> GPMGNGMNKILPGLYIGNFKDARDAEQLSKNKVTHILSVHDSARPMLEGVKYLCIPAADSPSQNLTRHFKESIKFIHECRLRGESCLVHCLAGVSRSVTLVIAYIMTVTDFGWEDALHTVRAGRSCANPAVGFQRQLQEFEKHEVHQYRQWLKE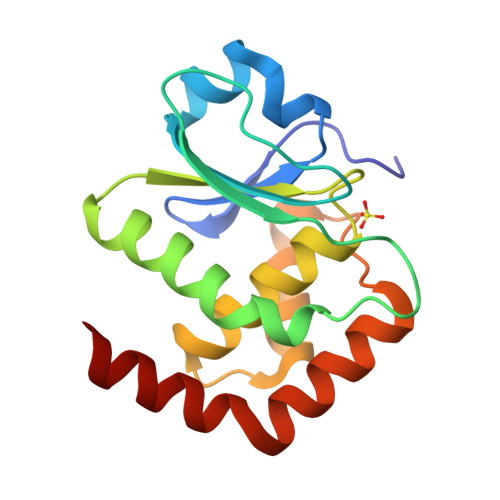EYG>MSTAIVTNVKHFGGMGSALRLSEAGHTVACHDESFKHQDELEAFAETYPQLIPMSEQEPVELIEAVT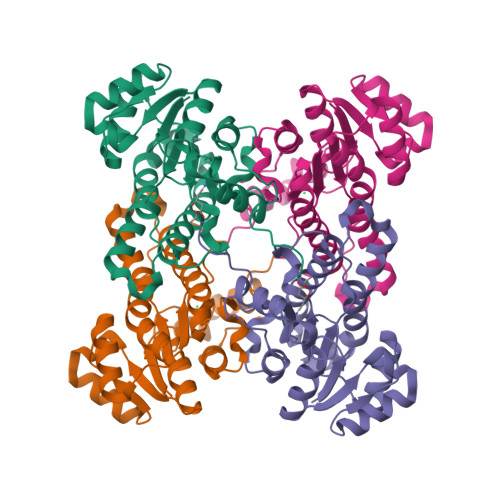SALGHVDILVSNDIAPVEWRPIDKYAVEDYRDMVEALQIKPFALANAVASQMKRRKSGHIIFITSAASFGPWKELSTYASARAGASALANALSKELGEHNIPVFAIAPNGVDSGDSPYYYPSEPWKTSPEHVAWVRKYTALQRLGTQKELGELVTFLASGSCDYLTGQVFWLAGGFPVVERWPGMPE[2x]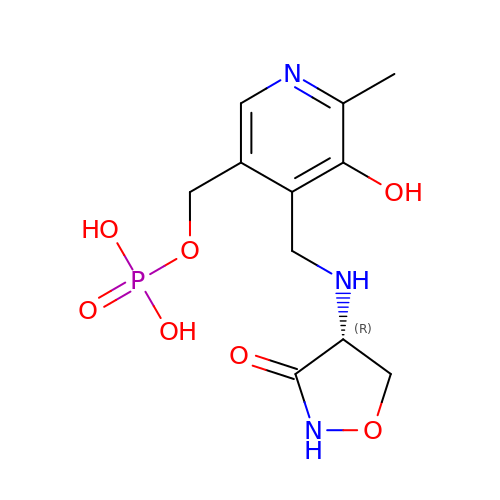D-[3-HYDROXY-2-METHYL-5-PHOSPHONOOXYMETHYL-PYRIDIN-4-YLMETHYL]-N,O-CYCLOSERYLAMIDE | C11 H16 N3 O7 P | NNRZSZJOQKAGTO-SECBINFHSA-N> GSHMDYNKRSSVSTVPNAAPIRVGFVGLNAAKGWAIKTHYPAILQLSSQFQITALYSPKIETSIATIQRLKLSNATAFPTLESFASSSTIDMIVIAIQVASHYEVVMPLLEFSKNNPNLKYLFVEWALACSLDQAESIYKAAAERGVQTIISLQGRKSPYILRAKELISQGYIGDINSIEIAGNGGWYGYERPVKSPKYIYEIGNGVDLVTTTFGHTIDILQYMTSSYFSRINAMVFNNIPEQELIDERGNRLGQRVPKTVPDHLLFQGTLLNGNVPVSCSFKGGKPTKKFTKNLVIDIHGTKRDLKLEGDAGFAEISNLVLYYSGTRANDFPLANGQQAPLDPGYDAGKEIMEVYHLRNYNAIVGNIHRLYQSISDFHFNTKKIPELPSQFVMQGFDFE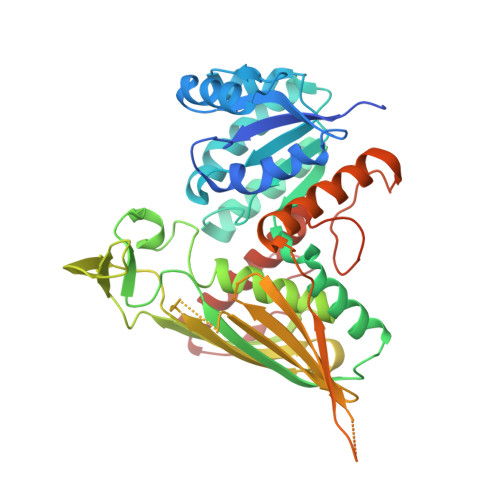GFPTLMDALILHRLIESVYKSNMMGSTLNVSNISHYSL>MAHHHHHHMPRIDLKTDKDFAELPEGTLAELLDGEIFMVPAPIPEHQRVIRKFSNALSTFVEKNKLGEVFFSPIDVYLDEHNVVQPDLIFISKARNTIIREKRIEGAPDWIAEILSEGNAYHDLKTKKRLYEKHGVAEYWIVDPMERSVEIYQNGNSGFTL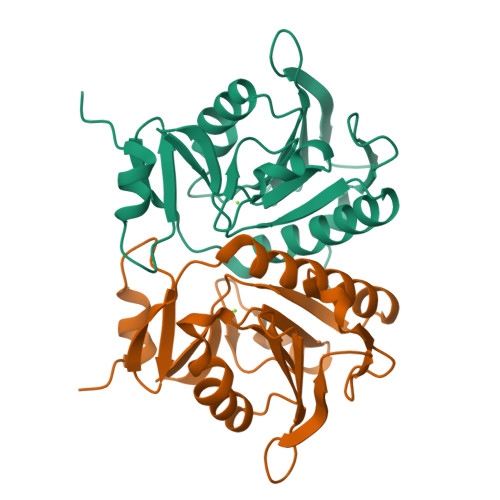LASADSGTVVSKMLDGFSLEIQTLFTKPL[2x]>MSAKQVSKDEEKEALNLFLSTQTIIKEALRKLGYPGDMYELMKEPQRMLTVRIPVKMDNGSVKVFTGYRSQHNDAVGPTKGGVRFHPEVNEEKVKALSIWMTLKCGIANLPYGGGKGGIICDPRTMSFGELERLSRGYVRAISQIVGPTKDIPAPDVYTNSQIMAWMMDEYSRLREFDSPGFITGKPLVLGGSQGRETATAQGVTICIEEAVKKKGIKLQNARIIIQGFGNAGSFLAKFMHDAGAKVIGISDANGGLYNPDGLDIPYLLDKRDSFGMVTNLFTDVITNEELLEKDCDILVPAAISNQITAKNAHNIQASIVVERANGPTTIDATKILNERGVLLVPDILASAGGVTVSYFEWVQNNQGYYWSEEEVAEK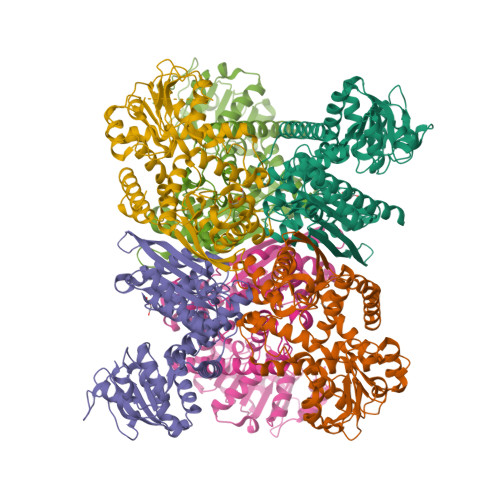LRSVMVSSFETIYQTAATHKVDMRLAAYMTGIRKSAEASRFRGWV[6x]> XWKQWKKY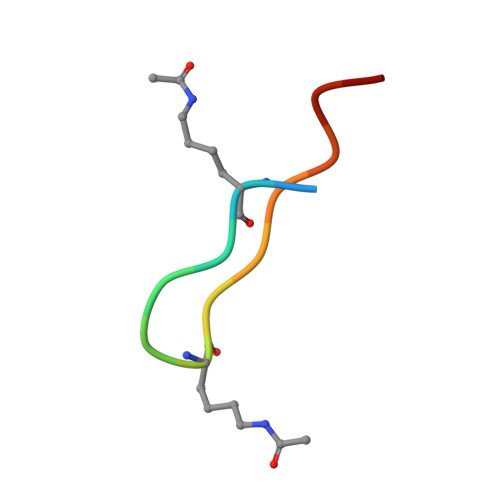GLKICX> VPSPYLLSDKEVREIVQQSLSVGNFAARMLVRLFPELFTTENLRLQYNHSGACNKKQLDPTRLRL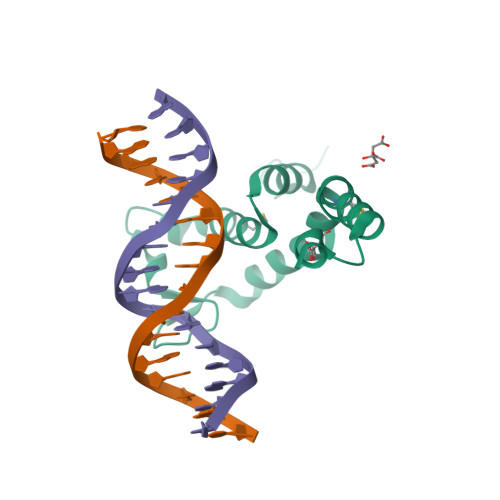IRHYVEAVYPVEKMEEVWHYECIPSIDERCRRPNRKKCDILKKAKKVEK>[2x]MIIERLVGNLRDLNPLDFSVDYVDLE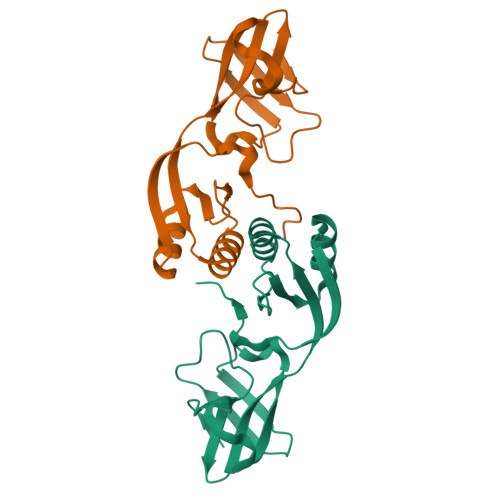WFETRKKIARFKTRQGKDIAIRLKDAPKLGLSQGDILFKEEKEIIAVNILDSEVIHIQAKSVAEVAKICYEIGNRHAALYYGESQFEFKTPFEKPTLALLEKLGVQNRVLSSKLDSKERLTVSMPHSEPNFKVSLASDFKVVVK>[2x]ALGVVGVLESYIGSINNITKQSACV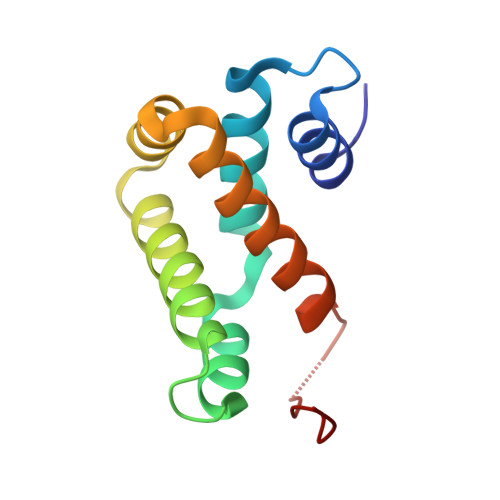AMSKLLTELNSDDIKKLRDNEELNSPKIRVYNTVISYIESNRKNNKQTIHLLKRLPADVLKKTIKNTLDIHKSITINNPKELTVSDTN>MSTLKNTFFITPPDTPTQAGPENIFYDFNDGARVLLPEGKWHVRLLDADSENILFCCDVDKGWVTSSKKYFVRFRIQVFRQGAATPLLDETLKLKDRPVLISFPTGTLGDLLGWFPYAERFQSLHKCRLECTMSQDIIDLLAPQYPQIQFSTPDKPRTVAPYATYRVGLYFGGDTNNQPVDFRKVGFHRSAGYILGVDPREAPVRLDLSAPRVIAAPYVCIATQSTCQAKYWNNGTGWSEVIAHLKSLGYRVMCIDRDAHYGQGFVWNHIPWGAEDFTGKLPLQERVNLLRHASFFIGLPSGLSWLAWATRIPVVLISGFSLPNSEFYTPWRVFNSHGCYGCWDDTSLNFDHHDFLWCPRHKNTDRQFECTRLITGAQVNGVINKLHRSLTEQGVEATLAAGVSNE[12x]

A subfamily of autotransporters, including AIDA-I (adhesin involved in diffuse adherence) from diffusely adhering E. coli (DAEC) 2787 and TibA from enterotoxigenic E. coli (ETEC) H10407, are glycosylated in their passenger domains, which functions in bacterial autoaggregation and adhesion to host cells. TibC catalyzes TibA/AIDA-I heptosylation and confers AIDA-I-mediated bacterial adhesion to host cells. Here we determine the crystal structures of TibC heptosyltransferase, both alone and in complex with ADP-D-glycero-β-D-manno-heptose (ADP-D,D-heptose). All the 12 TibC protomers adopt an identical structure containing an N-terminal β-barrel domain, a core catalytic domain, a β-hairpin thumb, and an iron-finger motif which are arranged into a palm-like shape.

A number of point mutations designed to reduce the surface entropy were screened and a TibC variant with three mutated epitopes (E83A/E84A, K400A/K401A, and Q215A/E216A) produced the highest quality crystal. This mutant exhibited identical biochemical and biological functions to wild-type TibC. Strikingly, one asymmetric unit in the solved structure contains 12 TibC molecules, which are assembled into a large ring structure. The overall shape of the dodecamer ring resembles a circular garland with an external diameter of 145 Å and a height of 72 Å. The inner surface of the stem is decorated with uniformly distributed 12 ferric ions, forming a characteristic iron belt along the ring. Six symmetric TibC protomers project upwards from the central plate while the other six project downwards, generating a gear-like shape at both sides. Two adjacent TibC protomers projecting oppositely contact each other in a back-to-back manner around a dyad axis; six back-to-back dimers are further linked together in a hand-in-hand fashion around a sixfold axis to form the garland-like ring. The β-hairpin thumb mediates the hand-in-hand contact between adjacent dimers. Within the module, a ferric ion is tetrahedrally coordinated by four conserved cysteine residues (Cys-339, 342, 358, and 370 in TibC), analogous to the zinc-finger motif. Thus, the iron finger is required for maintaining structural integrity of the TibC dodecamer.> NVVCVTGASG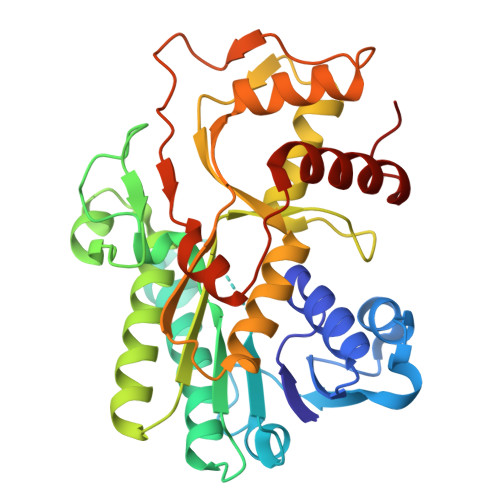YIASWLVRLLLHRGYTVKATVRDPNDPKKVDHLVKLDGAKERLQLFKANLLEEGAFDSVVQGCHGVFHTASPFYHDVKDPQAELIDPALKGTLNVLNSCAKSPSLKRVVLTSSIAAVAYNGKPRTPDVVVDETWFTDADFCAKSNLWYVVSATLAEEAAWKFVKENNIDMVTINPAMVIGPLLQPVLNTSAAAILNLINGAQTFPNASFGWVNVKDVANAHILAYENASASGRHCLVERVAHYSEVVRILRELYPSLQLPEKCADDKPYVPIYQVSKEKAKSLGLEYTPLEVSIKETVESLKEKKFANL> MVRKLK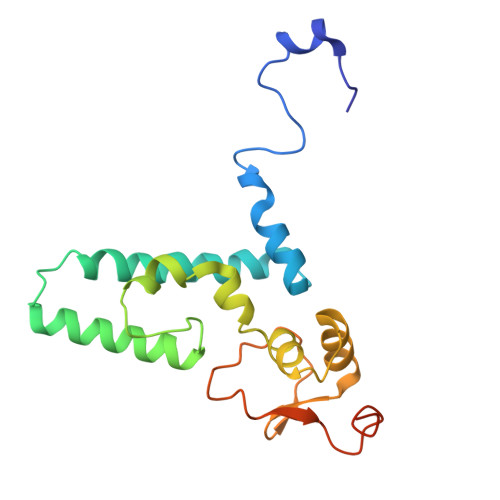HHEQKLLKKVDFLEWKQDQGHRDTQVMRTYHIQNREDYHKYNRICGDIRRLANKLSLLPPTDPFRRKHEQLLLDKLYAMGVLTTKSKISDLENKVTVSAICRRRLPVIMHRLKMAETIQDAVKFIEQGHVRVGPNLINDPAYLVTRNMEDYVTWVDNSKIKKTLLRYRNQIDDFDFS>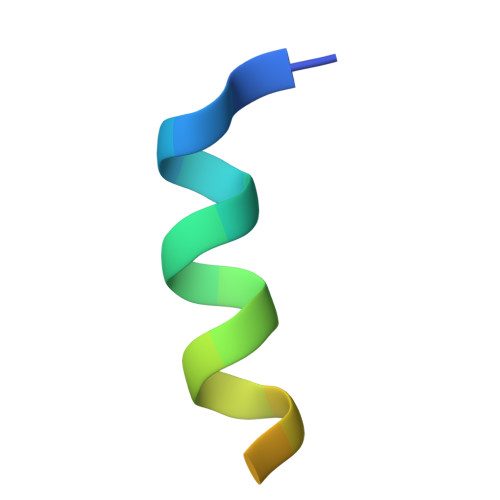 TNMGLEAIIRKALMGKYDQWEE> KNADSYAKKPHISALNAPQL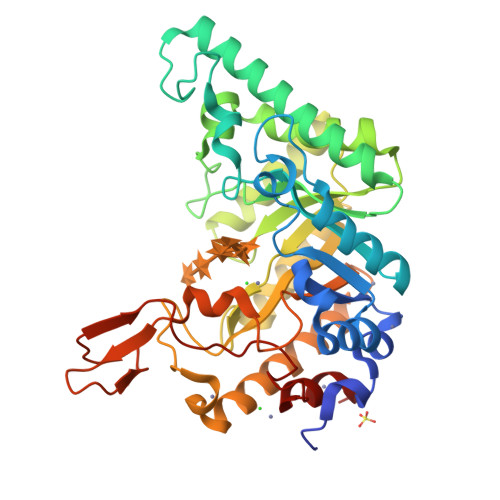DQRYKNEFTIGAAVEPYQLQNEKDVQMLKRHFNSIVAENVMKPISIQPEEGKFNFEQADRIVKFAKANGMDIRFHTLVWHSQVPQWFFLDKEGKPMVNETDPVKREQNKQLLLKRLETHIKTIVERYKDDIKYWDVVNQVVGDDGKLRNSPWYQIAGIDYIKVAFQAARKYGGDNIKLYMNDYNTEVEPKRTALYNLVKQLKEEGVPIDGIGHQSHIQIGWPSEAEIEKTINMFAALGLDNQITELDVSMYGWPPRAYPTYDAIPKQKFLDQAARYDRLFKLYEKLSDKISNVTFWGIADNHTWLDSRADVYYDANGNVVVDPNAPYAKVEKGKGKDAPFVFGPDYKVKPAYWAIIDHK>[2x]MDLIAPEDVVVTLSHAGYAKRQPVSAYRAQRRGGRGRSAASTKEEDFIDQLWLVNTHDTLLTFTSSGKVFWLPVHQLPEAGSNARGRPII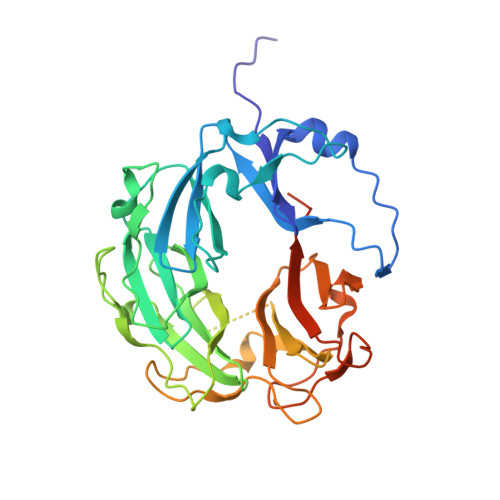NWIPLESGERVQAVLPVREYADNRYVFMATRNGTVKKTPLSEFAFRLARGKIAINLDEGDALVGVALTDGDRDVLLFASNGKTVRFGESTVRSMGRTATGVRGIRLAKGEEVVSLIVSERAGGVEDEVEDESAEEVVETTDGAEPAVIDVADNGDVAYILTATENGYGKRTPLAEYPRKGRGTQGVIGIQTTERNGKLVRAVLLGSTDEVMLISDGGTLVRTRGSEISRVGRNTQGVTLIRLSKGEKLQAVERLDASLEEPEDVVDEAVAITSDAPPAEG> MEAAHSKSTEECLAYFGVSETTGLTPDQVKRHLEKYGHNELPAEEGKSLWELVIEQFEDLLVRILLLAACISFVLAWFEEGEETITAFVEPFVILLILIANAIVGVWQERNAENAIEALKEYEPEMGKVYRADRKSVQRIKARDIVPGDIVEVAVGDKVPADIRILSIKSTTLRVDQSILTGESVSVIKHTEPVPDPRAVNQDKKNMLFSGTNIAAGKALGIVATTGVSTEIGKIRDQMAATEQDKTPLQQKLDEFGEQLSKVISLICVAVWLINIGHFNDPVHGGSWIRGAIYYFKIAVALAVAAIPEGLPAVITTCLALGTRRMAKKNAIVRSLPSVETLGCTSVICSDKTGTLTTNQMSVCKMFIIDKVDGDFCSLNEFSITGSTYAPEGEVLKNDKPIRSGQFDGLVELATICALCNDSSLDFNETKGVYEKVGEATETALTTLVEKMNVFNTEVRNLSKVERANACNSVIRQLMKKEFTLEFSRDRKSMSVYCSPAKSSRAAVGNKMFVKGAPEGVIDRCNYVRVGTTRVPMTGPVKEKILSVIKEWGTGRDTLRCLALATRDTPPKREEMVLDDSSRFMEYETDLTFVGVVGMLDPPRKEVMGSIQLCRDAGIRVIMITGDNKGTAIAICRRIGIFGENEEVADRAYTGREFDDLPLAEQREACRRACCFARVEPSHKSKIVEYLQSYDEITAMTGDGVNDAPALKKAEIGIAMGSGTAVAKTASEMVLADDNFSTIVAAVEEGRAIYN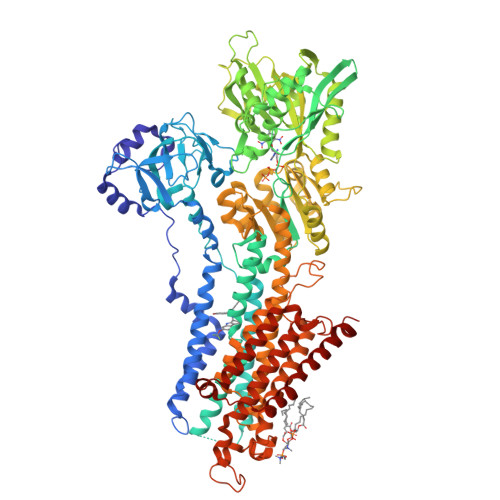NMKQFIRYLISSNVGEVVCIFLTAALGLPEALIPVQLLWVNLVTDGLPATALGFNPPDLDIMDRPPRSPKEPLISGWLFFRYMAIGGYVGAATVGAAAWWFMYAEDGPGVTYHQLTHFMQCTEDHPHFEGLDCEIFEAPEPMTMALSVLVTIEMCNALNSLSENQSLMRMPPWVNIWLLGSICLSMSLHFLILYVDPLPMIFKLKALDLTQWLMVLKISLPVIGLDEILKFIARNYLEG>MSKYEGRWTTVKVELEAGIAWVTLNRPEKRNAMSPTLNREMVDVLETLEQDADAGVLVLTGAGESWTAGMDLKEYFREVDAGPEILQEKIRREASQWQWKLLRLYAKPTIAMVNGWCFGGGFSPLVACDLAICANEATFGLSEINWGIPPGNLVSKAMADTVGHRQSLYYIMTGKTFDGRKAAEMGLVNDSVPLAELRETTRELALNLLEKNPVVLRAAKNGFKRCRELTWEQNED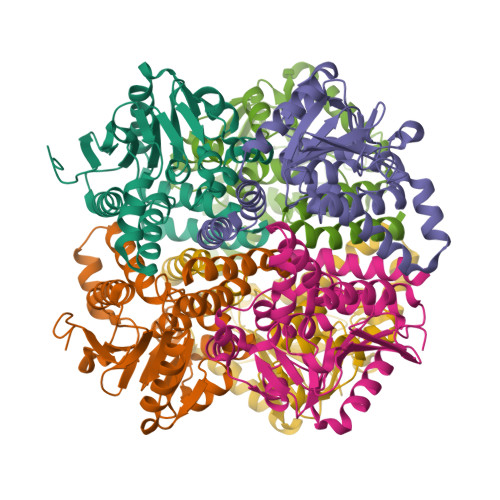YLYAKLDQSRLLDTTGGREQGMKQFLDDKSIKPGLQAYKRLEHHHHHH[2x]>[4x]MKLAVYSTKQYDKKYLQQVNEAFGFELEFFDFLLTEKTAKTANGCEAVCIFVNDDGSRPVLEELKKHGVKYIALRCAGFNNVDLD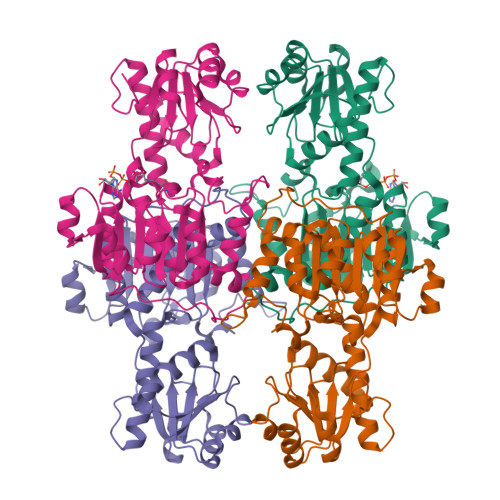AAKELGLQVVRVPAYSPEAVAEHAIGMMMTLNRRIHRAYQRTRDANFSLEGLTGFTMHGKTAGVIGTGKIGVAALRILKGFGMRLLAFDPYPSTAALDLGVEYVDLQTLFAESDVISLHCPLTPENYHLLNHAAFDQMKNGVMIINTSRGALIDSQAAIEALKNQKIGSLGMDVYENERDLFFEDKSVDVIQDDVFRRLSACHNVLFTGHQAFLTAEALISISETTLQNLSQLEKGEACPNALFKHHHHHHHH>[2x]ETGGLLNCPIYWQQLREKCLLFSHTVNPWNNSLADCSTKESSLLLI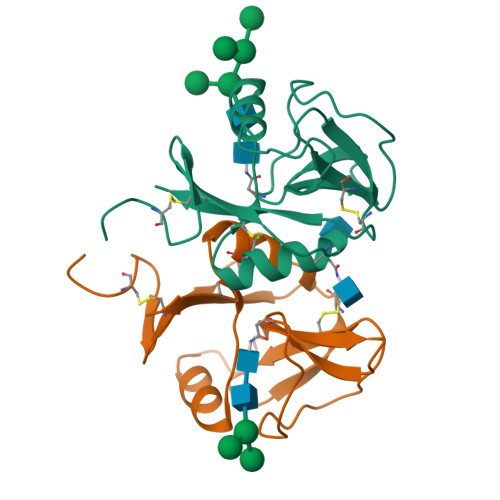RDKDELIHTQNLIRDKAILFWIGLNFSLSEKNWKWINGSFLNSNDLEIRGDAKENSCISISQTSVYSEYCSTEIRWICQKELTPVRNKVYPDSKHHHHHH> MKDYDELLKYYELHETIGTGGFAKVKLACHILTGEMVAIRIMDKNTLGSDLPRIKTEIEALKNLRHQHICQLYHVLETANKIFMVLEYCPGGELFDYIISQDRLSEEETRVVFRQIVSAVAYVHSQGYAHRDLKPENLLFDEYHKLKLIAFGLCAKPKGNKDYHLQTCCGSLAYAAPELIQGKSYLGSEADVWSMGILLYVLMCGFLPFDDDNVMALYKKIMRGKYDVPKWLSPSSILLLQQMLQVDPKKR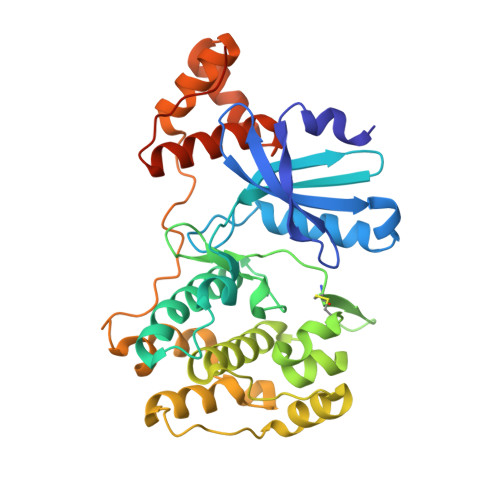ISMKNLLNHPWIMQDYNYPVEWQSKNPFIHLDDDCVTELSVHHRNNRQTMEDLISLWQYDHLTATYLLLLAKKARGKPVRLRLSSFSCGLEHHHHHH>[8x]MATQGVFTLPANTRFGVTAFANSSGTQTVNVLVNNETAATFSGQSTNNAVIGTQVLNSGSSGKVQVQVSVNGRPSDLVSAQVILTNELNFALVGSEDGTDNDYNDAVVVINWPLG;>K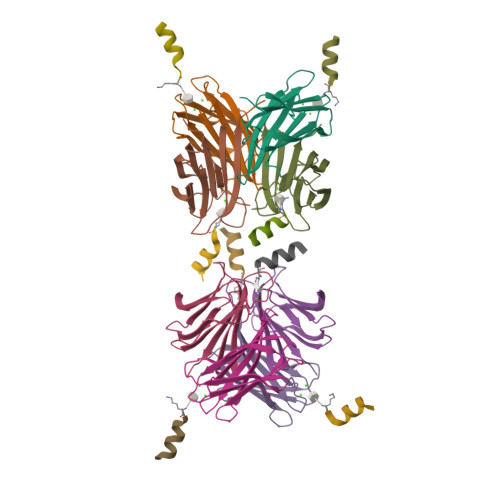KLLKLLKLLLX[8x]2-(4-hydroxyphenyl)-~{N}-methyl-5-oxidanyl-4-(piperidin-1-ylmethyl)-1-benzofuran-3-carboxamide 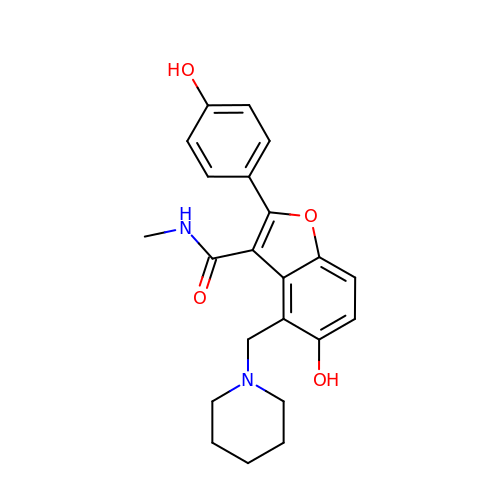| C22 H24 N2 O4 | PQGCMFVNJWTUFH-UHFFFAOYSA-N>MPTDLERRRAIDTAASMYLAEEPLDMSLLAERLGVGRATLYRWVGNRDELLGTVLAEATERTYRKAMSQASGQGPEYILDVFGRVMRSVESSTELRALTKREPMVFIKLAMMPGSIESISASITAEILQSQVDAGQLTITLSPQVLGEALVRICDVHLYAPLLGREKAEIETALDLIALLLGVTRNHHHHHH[2x]

In R. erythropolis, the lactonase QsdA has been identified as the only lactonase. We named the incriminated gene qsdR (quorum-sensing degradation regulation) which codes for a transcriptional regulator of the TetR/FabR family. QsdR protein possesses a DNA-binding domain at the N-terminus and a regulatory domain at the C-terminus. The DNA-binding domain permits the protein to bind DNA inducing genes activation or repression under its control.

QsdR shares low sequence identity (around 20%) with regulatory proteins with known three dimensional structures. Thus the structure of QsdR at 2.4 Å resolution was solved using sulfur SAD method. A better resolution structure at 1.9 Å of QsdR from a different crystallization condition was determined by molecular replacement (using the sulfur-SAD structure as model) with two identical molecules in the asymmetric unit (root mean square deviation (rmsd) of 0.07 Å for 181 Cα atoms). Each molecule of QsdRwt comprises 186 residues and is composed of 11 α helices, 3 of them corresponding to the DNA-binding domain, and the others to the regulatory domain. The DNA-binding domain (residues 2 to 41) forms the N terminus domain while the regulatory domain (residues 47 to 186) constitutes the C terminus. These two domains are connected by two residues, Glycine 45 and Asparagine 46. Each monomer in the asymmetric unit forms a dimer by the crystallographic symmetry. The dimer interface covers 995 A2 per subunit involving 19 residues located in helices α7, α 9 and α10 and two loops, one between α7 and α8 and the other between α9 and α10. Therefore, the dimeric structure of QsdRwt is the functional form in solution in line with results from gel filtration chromatography (molecular mass estimates at 44 kDa). The regulatory domain of QsdR presents a half hydrophobic/half polar cavity suggesting that QsdR can bind molecules having both hydrophobic and polar groups such as NAHL.>MSVRRTKIVATLGPASNSPEVLEQLILAGIDVARLNFSHGTPDEHRARARLVRELAAKHGRFVALLGDLQGPKIRIAKFANKRIELQVGDKFRFSTSHARDAGTQEVVGIDYPDLVKDCGVGDELLLDDGRVVMVVEEVAADELRCRVLIGGPLSDHKGINRRGGGLTAPALTDKDKADIKLAADMDLDYVAVSFPRDAKDMEYARRLLTEAGGKAWLVAKIERAEAVADDDALDGLIRASDAVMVARGDLGVEIGDAELVGIQKKIILHARRNNKVVITATQMMESMIHSPMPTRAEVSDVANAVLDYTDAVMLSAESAAGEYPVEAVKAMARVCQGAEKHPTSQKSSHRLGQTFDRCDESIALASMYTANHFPGIKAIICLTESGFTPLIMSRIRSSVPIYAYSPHRETQARVAMFRGVETIPFDPAALPAEKVSQAAVDELLKRGVVTKGDWVILTKGDSYTAQGGTNTMKVLHVGDLLV[12x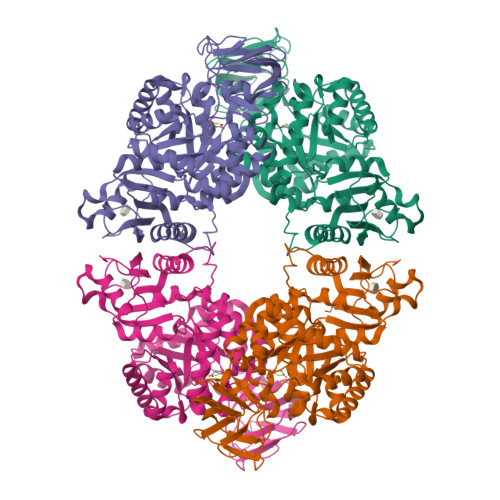]META-TYROSINE | C9 H11 N O3 | 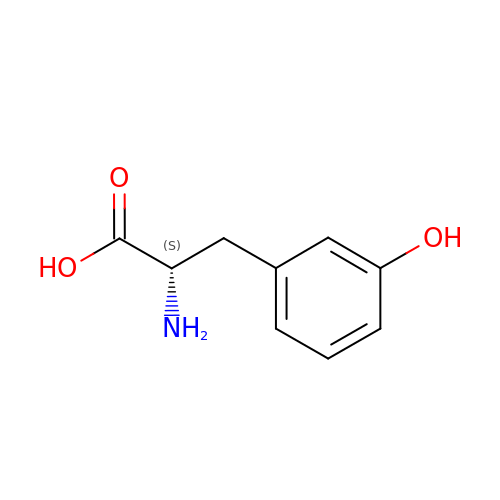JZKXXXDKRQWDET-QMMMGPOBSA-N The periplasmic ligand binding proteins (PLBPs) recognize diverse ligands and deliver their cargo to membrane-bound members of the ABC-type family for selective uptake into the cytoplasm. However, structures of metal binding PLBPs of cluster 9 family display a distinct fold wherein a rigid α-helix connects the two terminal domains. Towards this end, we have determined the crystal structure of native (non-recombinant) ZnuA from E. coli in a naturally zinc bound state. Superposition of the two independent molecules in the asymmetric unit yields a root-mean-square deviation (r.m.s.d.) value of 0.3 Å for 933 backbone atoms and therefore we are, for the most part, presenting and discussing molecule A. Structure of ZnuA-Ec possesses a pair of (α/β)4 sandwich domains which are held together by a long linker α helix that is tightly packed against them.

The asymmetric unit is composed two protomers of ZnuA (molecules A and B; 520 residues), and includes two zinc ions and 527 water molecules. The metal binding pocket in ZnuA-Ec is formed at the interface of the N and C-domains. Zinc is coordinated by residues His60, His143, His207 and a water molecule. While the histidine residues coordinate zinc via Nε2 atoms in a trigonal pyramid geometry, the fourth ligand water occupies the apical position. Interestingly, Glu59, which is close to the active site water, makes a direct long coordination bond with Zn2+ (2.8 Å in molecule A and 3.3 Å in molecule B). Intriguingly, however, ZnuA-Ec possesses a unique disulfide bond (Cys252–Cys306) in an unexpected location, between strand G and helix h. This disulfide bond is surface exposed, and is a novel feature of ZnuA-Ec, as it is absent from homologous zinc transporters. However, in ZnuA-Ec, which we propose presents a snapshot of the bound state, there is no equivalent water. Instead, we propose a “partial domain slippage” mechanism which stems from small yet significant conformational changes in multiple locations of ZnuA, which together potentially drive binding and release of zinc. In this light, we assign the present ZnuA-Ec complex with zinc as the metal “bound” state while other previous structures like ZnuA-Syn may represent initial conformational steps of the metal “release” state.

>[2x]MLHKKTLLFAALSAALWGGATQAADAAVVASLKPVGFIASAIADGVTETEVLLPDGASEHDYSLRPSDVKRLQNADLVVWVGPEMEAFMQKPVSKLPGAKQVTIAQLEDVKPLLMKSIHGDDDDHDHAEKSDEDHHHGDFNMHLWLSPEIARATAVAIHGKLVELMPQSRAKLDANLKDFEAQLASTETQVGNELAPLKGKGYFVFHDAYGYFEKQFGLTPLGHFTVNPEIQPGAQRLHEIRTQLVEQKATCVFAEPQFRPAVVESVARGTSVRMGTLDPLGTNIKLGKTSYSEFLSQLANQYASCLKGD>[6x]MLTKQAVEPVRINARTTDVFDIFNVKQYVGANPYLNQAALVFDFAFTESYQPLPIENYLAVVGDRYPRLKEIEYQSYAELFASTVAEVNKLEMDLHLKGWNVKPIEEINRIAIESLHHRTTKEVVYCVWDWFEFITQGEEFDLSKQIAILQQLFRNSVYG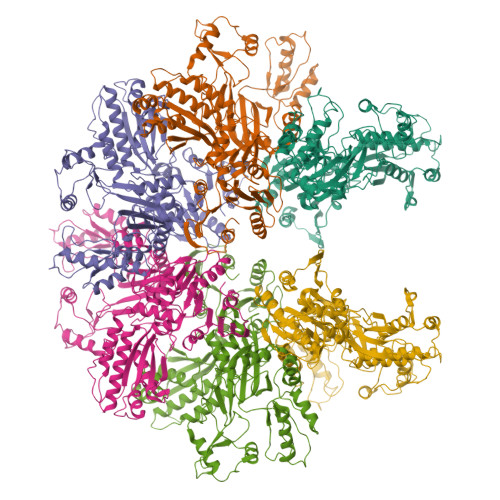GPTVYALLRTANEKHIPAFYLWDEGLMQYGYGKQQVRGIATTFDVDSHIDSDFTTQKDDCKKFLQELGFPVPQGDVVFSLAEAKEVAAEIGYPVAVKPVAGHKGIGVTADVQDEIELEAAYDRAVAGIPLEEKICIIVENSIAGHDYRLLCVNGRFVAATERKPAYVVGDGYSTIAELIEKENFSPNRSDTPTSPMGKIRTDEAMHLYLEEQGLDLDSVIDRDRTIYLRKVANLSSGGFSIDATNRVHPDNIILAQDIAQHFRLTCLGIDIITNDIGRSWKETSFGIIEINAAPGVYMHLKPAIGEPVDVTARILETFFETEKNARIPIITFNRVSIRQLQKLSDRILMSHPDWTIGAVCREGILINRSEKILNRHYNTNVLNLLRNPKLDLLIAEYDEDALEAEGMFYHGSNLVVLEDPSEIEMILTRDVFSDSTVIIKQGREITIKRKGLLEQYELEAEELIEQVYLKEIGTISENLYFQ>[2x]GHMAKTYDYLFKLLLIGDSGVGKTCVLFRFSEDAFNSTFISTIGIDFKIRTIELDGKRIKLQIWDTAGQERFRTITTAYYRGAMGIMLVYDITNEKSFDNIRNWIRNIEEHASADVEKMILGNKCDVNDKRQVSKERGEKLALDYGIKFMETSAKANINVENAFFTLARDIKAKMDKKLEGNSPQG;>GPGYERLKEELAKAQ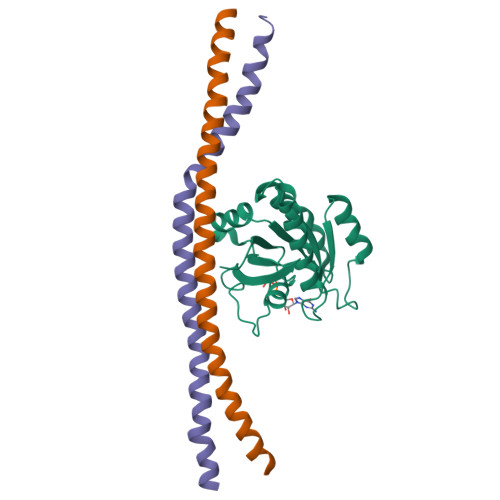RELKLKDEECERLSKVRDQLGQELEELTASLFEEAHKMVREANIKQATAEKQLKEAQGKIDVL[4x]The hypothetical protein ORF6 of the Enc34 phage is conserved among all Nazgul-like phages and consists of a single domain, currently annotated as a domain of an unknown function DUF2815. Here, we present structural and functional characterization of the Enc34 ORF6 that allows us to establish its function as a single-stranded DNA-binding protein (SSB) and extend this annotation to other DUF2815 family members. The SSBs are ubiquitous within all kingdoms of life and in DNA viruses, and protect ssDNA intermediates during replication, repair and recombination. In this study, we show that the Enc34 ORF6 is structurally homologous to the gene 2.5 protein from bacteriophage T7, and present a high-resolution structure of ORF6 in complex with ssDNA, which reveals for the first time the structural basis for the ssDNA-binding mechanism of T7-type SSBs.

The structure of the full-length Enc34 ORF6 protein was solved to 1.50 Å resolution using a selenomethionine-substituted protein. The model contains a single protein chain with 179 modeled residues; the very first N-terminal and eleven C-terminal residues of the full-length protein were not visible in the electron density map due to disorder, and two loop regions (residues 39–43 and 98–100), were also poorly structured and therefore not included in the final model. Apart from the C-terminus, the Enc34 ORF6 protein adopts a compact, roughly globular shape with a diameter of approximately 40 Å and has a mixed α/β architecture comprised predominantly of β-strands. The protein can be regarded as built up from a concave seven-stranded β-sheet at one side of the protein, of which the three central strands together with the two β-strands from the opposite side form a slightly flattened five-stranded β-barrel at the protein core, and two α-helices cap the β-barrel at both ends. The ORF6 structure extends from the canonical OB-fold by having two extra strands (β1′ and β1″) at the N-terminus, a helix α1 and strand β23′ in the loop connecting β2 and β3, and two extra strands β34′ and β34″ between β3 and helix α2. The helix α1 is rather long and packs with the three N-terminal strands, completely obstructing the opening of the β-barrel. The C-terminus of the ORF6 protein is notably acidic with 16 of the 29 C-terminal residues being either aspartates or glutamates. These residues, as far as they are visible in the electron density map, do not form any secondary structure and extend away from the rest of the protein in a direction nearly parallel to strands β4 and β5. Interestingly, the very end of the traceable C-terminus inserts into the groove of the seven-stranded β-sheet of a neighboring molecule in the crystal, with possible implications for oligomerization.

> GLAEKLVPAKKVKNGVLYKSGHIKVSNVRCSYPHLDKPYGGEDGGEPKYSITLLMPKDTHGAIKKIIDEQIELTKKNHKTGALKVAPSMLFIKDGDVDFPDKPECEGMWVISARESTRPDVLNMEREELESPNEIAEEIYGGCWVSSVIRPWSQENKYGKRINANLLSVLKRKDDEPFGEGRVDTSDAYDEDEDEWDEDEV>[3x]MTKVALFSGGDLTYFTRD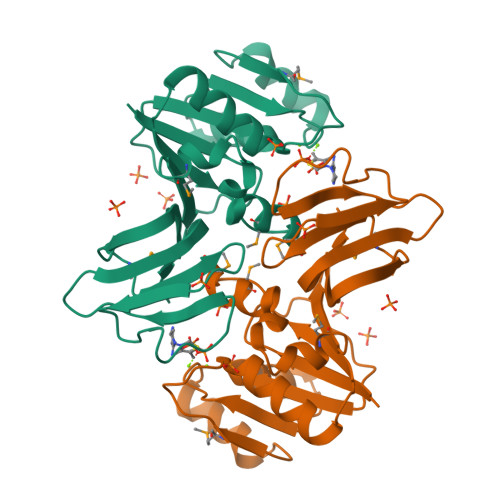FDYFVGIDKGSSFLLKNQLPLDLAIGDFDSVSAEEFKQIKAKAKKLVMAPAEKNDTDTELALKTIFDCFGRVEIIVFGAFGGRIDHMLSNIFLPSDPDLAPFMRCFKLRDEQNLVEFFPAGQHQIEQATDMVYISFMAANGAHLSIQDAKYELTEENYFQKKIYSSNEFKDKPICFSVASGYVVVIQTKDRTLEHHHHHH>[4x]MRGSHHHHHHGSIEGRMEKINYLLPEESAEMTLNQVKSLRQIEGRLRKLFSLKNYQEVMPPSFEYTQLYTALESNGKTFNQEKMFQFIKHEGQSITLRYDFTLPLVRLYSQIKDSTSARYSYFGKIFRKEKRHKGRSTENYQIGIELFGESADKSELEILSLALQVIEQLGLNKTVFEIGSAKFFQRLCQLADGSTELLTELLLKKDLSGLNAFIEKNNFSKELRGLLKEIFITNELSRLENLVTNTKDDVLISSFDQLKEFSEKLSMIKPIIIDLGMVPKMDYYTDLMFKAYSSAANQPILSGGRYDQLLSNFQEEAFAIGFCCHMDTILKALERQELEEDND;>MIKIAITKGRIQKQVTKLLENADYDVEPILNLGRELQIKTKDDLQIIFGKPNDVITFLEHGIVDIGFVGKDTL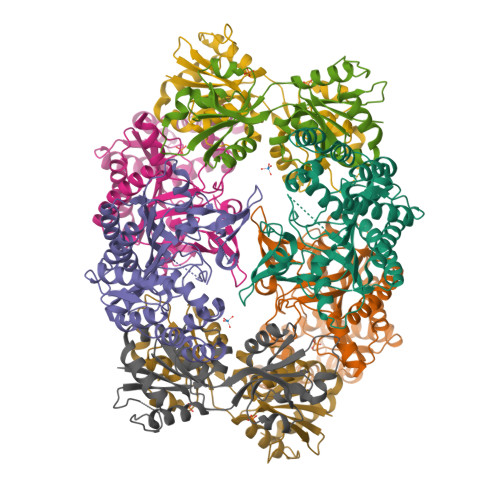DENDFDDYYELLYLKIGQCIFALASYPDFSNKNFQRHKRIASKYPRVTKKYFAQKQEDIEIIKLEGSVELGPVVGLADAIVDIVETGNTLSANGLEVIEKISDISTRMIVNKSSFKFKKDKIIEMVERLEDAQTN[4x]> GASRASRSHSRREEHSGRNGLHHPSPDHFWPRFPDALRPFVPWDQLENEDSSVHISPRQKRDANSSIYKGKKCRMESCFDFTLCKKNGFKVYVYPQQKGEKIAESYQNILAAIEGSRFYTSDPSQACLFVLSLDTLDRDQLSPQYVHNLRSKVQSLHLWNNGRNHLIFNLYSGTWPDYTEDVGFDIGQAMLAKASISTENFRPNFDVSIPLFSKDHPRTGGERGFLKFNTIPPLRKYMLVFKGKRYLTGIGSDTRNALYHVHNGEDVVLLTTCKHGKDWQKHKDSRCDRDNTEYEKYDYREMLHNATFCLVPRGRRLGSFRFLEALQAACVPVMLSNGWELPFSEVINW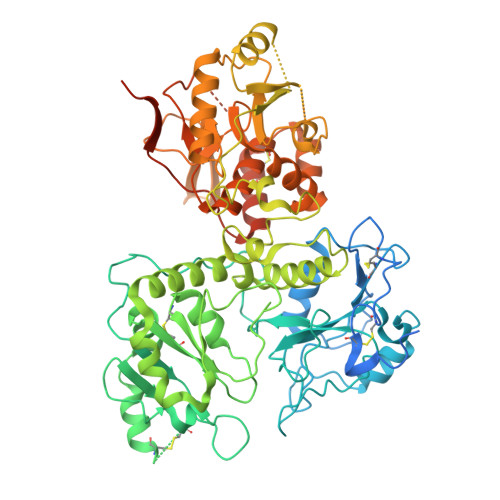NQAAVIGDERLLLQIPSTIRSIHQDKILALRQQTQFLWEAYFSSVEKIVLTTLEIIQDRIFKHISRNSLIWNKHPGGLFVLPQYSSYLGDFPYYYANLGLKPPSKFTAVIHAVTPLVSQSQPVLKLLVAAAKSQYCAQIIVLWNCDKPLPAKHRWPATAVPVVVIEGESKVMSSRFLPYDNIITDAVLSLDEDTVLSTTEVDFAFTVWQSFPERIVGYPARSHFWDNSKERWGYTSKWTNDYSMVLTGAAIYHKYYHYLYSHYLPASLKNMVDQLANCEDILMNFLVSAVTKLPPIKVTQKKQYKETMMGQTSRASRWADPDHFAQRQSCMNTFASWFGYMPLIHSQMRLDPVLFKDQVSILRKKYRDIERLNNNNNNGHHHHHHHH> MWIPVVGLPRRLRLSALAGAGRFCILGSEAATRKHLPARNHCGLSDSSPQLWPEPDFRNPPRKASKASLDFKRYVTDRRLAETLAQIYLGKPSRPPHLL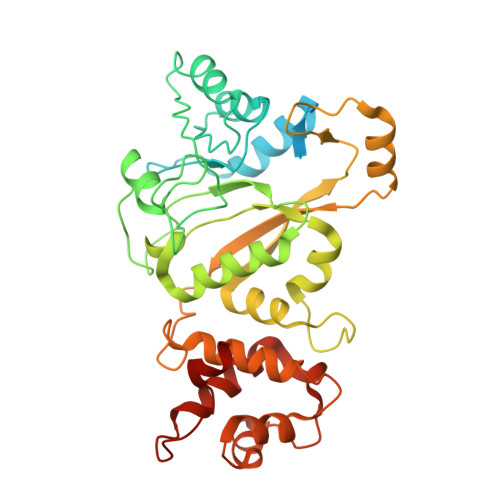LECNPGPGILTQALLEAGAKVVALESDKTFIPHLESLGKNLDGKLRVIHCDFFKLDPRSGGVIKPPAMSSRGLFKNLGIEAVPWTADIPLKVVGMFPSRGEKRALWKLAYDLYSCTSIYKFGRIEVNMFIGEKEFQKLMADPGNPDLYHVLSVIWQLACEIKVLHMEPWSSFDIYTRKGPLENPKRRELLDQLQQKLYLIQMIPRQNLFTKNLTPMNYNIFFHLLKHCFGRRSATVIDHLRSLTPLDARDILMQIGKQEDEKVVNMHPQDFKTLFETIERSKDCAYKWLYDETLEDR>MSGSHHHHHHSGSMSERPSDLVVNRLVLFVVKGTATSTHNTVKPLILLEELGVPHDIYVVEKVSAPWFSEINPHKMVPAILDRSPDGRDTLRAWEATSTLMYIADAYDKDGTFGGRNVQERSEINNWLTLHTAALGPTAKYWLYFYKLHPEKLPKTIEKLRSNITVQYDILERRLNEPGQQYLALKDRPTIADIATLPFAMKSTAELFGLEFEKWPKLQEWSVRMGEREAVKRAWQRVAG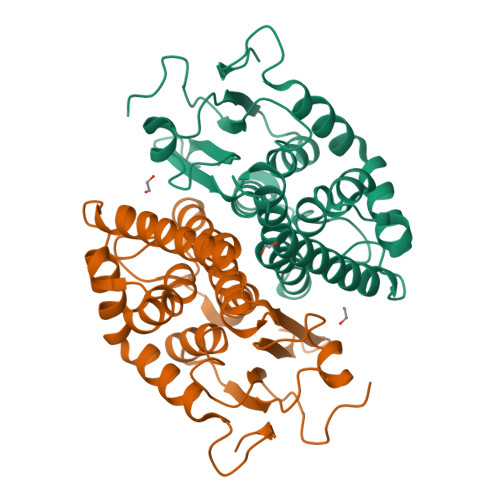FGHGEKEYGMLEA[6x]>DEKVVDEVKYS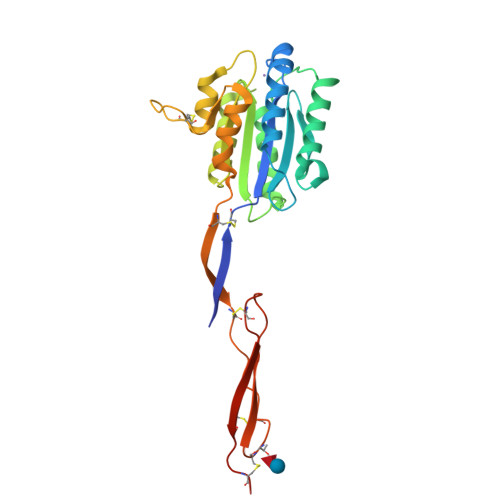EEVCNEQVDLYLLVDGSGSIGYPNWITKVIPMLNGLINSLSLSRDTINLYMNLFGSYTTELIRLGSGQSIDKRQALSKVTELRKTYTPYGTTSMTAALDEVQKHLNDRVNREKAIQLVILMTDGVPNSKYRALEVANKLKQRNVRLAVIGIGQGINHQFNRLIAGCRPREPNCKFYSYADWNEAVALIKPFIAKVCTEVERVANCGPWDPWTACSVTCGRGTHSRSRPSLHEKCTTHMVSECEEGECPHHHHHHA[2x]tert-butyl [(2R,3S)-1-(1,4-dimethyl-2-oxo-1,2-dihydroquinolin-7-yl)-6-oxo-2-phenylpiperidin-3-yl]carbamate 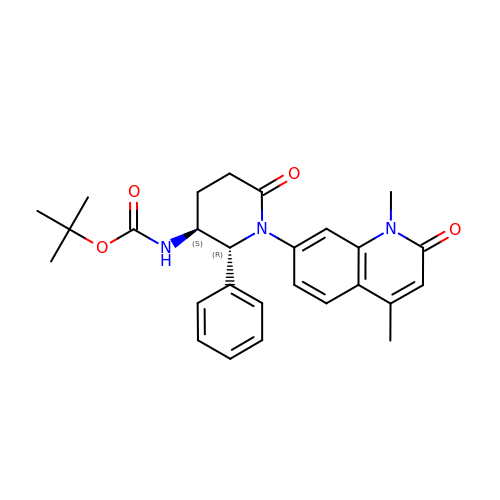| C27 H31 N3 O4 | SMDVXOGKDHVOGV-SQJMNOBHSA-N> AKREPIHDNSIRTEWEAKIAKLTSVDQATKFIQDFRLAYTSPFRKSYDIDVDYQYIERKIEEKLSVLKTEKLPVADLITKATTGEDAAAVEATWIAKIKAAKSKYEAERIHIEFRQLY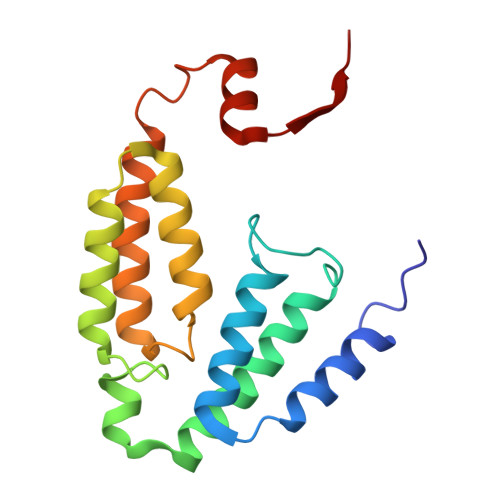KPPVLPVNVFLRTDAALGTVLMEIRNTDYYGTPLEGLRKERGVKVLHLQA>[8x]MSAQRAYNFSAGPAAVPLECLERAAAEMTNWRNSGMSVIEVSHRGKHWMEEQKEATERLRTLLQVPENFNILFVAGGASLQFSAIPFNFIGEHKAVDYLCTGTWSKKAFDECKRLAFPGVTVNSVAGNPPANPVEVPARDTWKLSEDAAYFYYCDNETIQGIEFQQFPDVPAPLIIDMSSNFLSRPITQWEKVGCIFACAQKNFGLAGMSVVIIRKDMLERPVKPFCPIT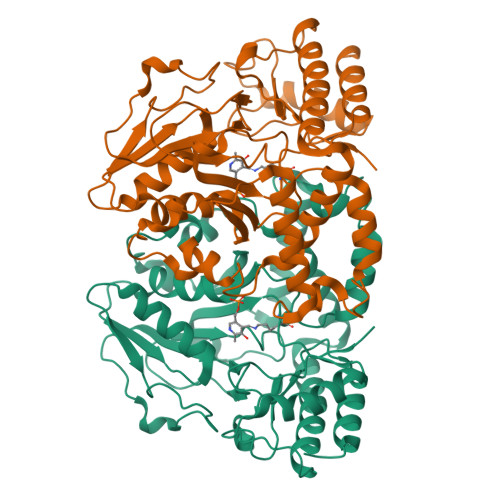MDYRIQVKNNCMYNTPPTFAIYFANHIFKWIEEKGGLAAMDALNKEKAKKVYEAIDSNPNFVNRIKPEWRSRMNMPFFRPDGYENKDLDADAKFVNFCTQRKLLTLKGHVSVGGFRASCYNACPMEAVDALVQAMKEWPGFLEHHHHHH>GPLGSEVYKGDGYKVWKLEPSLGDPLELGRKTKTEMNAMTHDEFDRMKYRGVVAEVYSGDKPSKGYDKLRVLLDLMDRPRLGTTVDLCAGRGGWSELVKDLEGPKGITAVSLWERGKEEWMADPAIHRINANVKHLRPWQVDTLLFDGGEAFKRDQNLRKEENFNDSLLDAVDAWMMQPVPPRNFVIKIQVPYTQKAIALLEKWQVKTGKGRLVRLAGDRLSNTVMYFLSVRLETQIRGRVTTFVRELAERRKDRSLTADPSLQYERVEPQWTEEAR[2x]

Alongshan virus (ALSV), a newly discovered member of unclassified Flaviviridae family, is able to infect humans. ALSV NSP1 is a typical flavivirus NS5-like protein. It carries two essential enzymatic activities: the methyltransferase (MTase) and the RNA-dependent RNA polymerase (RdRp). The flaviviral NS5-MTase functions to catalyze the methylation of viral RNA cap.

The crystal structure of apo ALSV MTase was determined using the single-wavelength anomalous dispersion method and finally refined to a resolution of 2.5 Å, with Rwork and Rfree values of 0.209 and 0.258, respectively. Clear electron densities could be observed for residues E42-K84, S99-W149 and E155-A295. Amino acids Y85-P98, E150-E154 and D296-R313, however, were unable to be traced due to high flexibility. Overall, the ALSV enzyme has a globular fold, which can be further divided into three subdomains (the N-terminal and C-terminal extension regions and the core region). The N-terminal extension region consists of an extended loop followed by a helix-turn-helix motif (helices A1 and A2). The core region folds into a seven stranded β-sheet (strands β1-β7) surrounded by four α helices (helices αX, αA, αD and αE), which reveals the general αβα-Rossmann-fold. The C-terminal extension region consists mainly of an α-helix (helix A3). The overall structure of ALSV MTase is similar to those of the MTase proteins from canonical unsegmented flaviviruses. For ALSV MTase, it contained a long-extended N-terminal loop, which was not present in DENV3 MTase. In addition, following the helix-turn-helix motif in the N-terminal extension, the ALSV enzyme also featured with a shortened loop that is highly flexible (amino acids Y85-P98 being untraceable in the electron density map).> MLQFYRNLGKSGLRVSCLGLGTWVTFGGQITDEMAEHLMTLA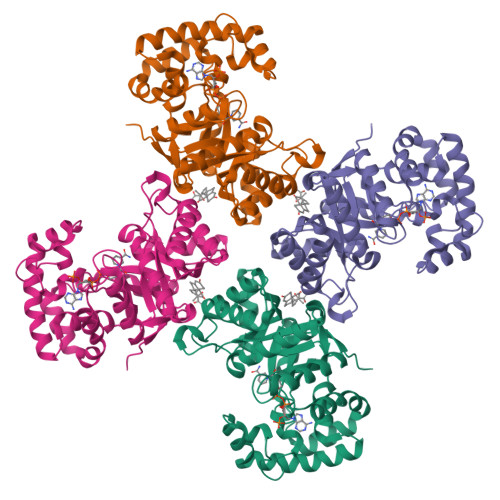YDNGINLFDTAEVYAAGKAEVVLGNIIKKKGWRRSSLVITTKIFAGGKAETERGLSRKHIIEGLKASLERLQLEYVDVVFANRPDPNTPMEETVRAMTHVINQGMAMYWGTSRWSSMEIMEAYSVARQFNLIPPICEQAEYHMFQREKVEVQLPELFHKIGVGAMTWSPLACGIVSGKYDSGIPPYSRASLKGYQWLKDKILSEEGRRQQAKLKELQAIAERLGCTLPQLAIAWCLRNEGVSSVLLGASNAEQLMENIGAIQVLPKLSSSIVHEIDSILGNKPYS> SQDDEFCRVIPTVRKAKLLPMEEAL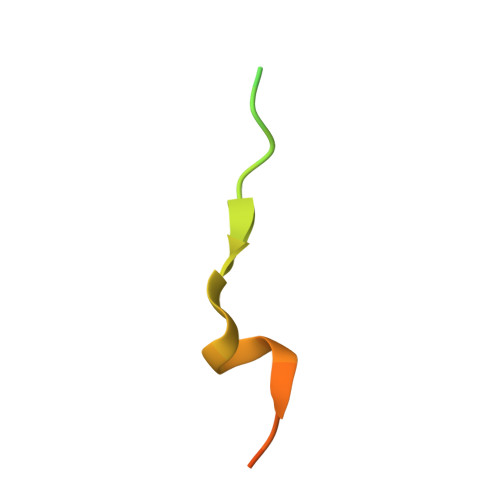LPAPTFTQ>STAGKVIKCKAAVLWEEKKPFSIEEVEVAPPKAHEVRIKMVATGICRSDDHVVSGTLVTPLPVIAGHEAAGIVESIGEGVTTVRPGDKVIPLFTPQCGKCRVCKHPEGNFCLKNDLSMPRGTMQDGTSRFTCRGKPIHHFLGTSTFSQYTVVDEISVAKIDAASPLEKVCLIGCGFSTGYGSAVKVAKVTQGSTCAVFGLGGVGLSVIMGCKAAGAARIIGIDINKDKFAKAKEVGATECVNPQDYKKPIQEVLTEMSNGGVDFSFEVIGRLDTMVTALSCCQEAYGVSVIVGVPPDSQNLSMNPMLLLSGRTWKGAIFGGFKSKDSVPKLVADFMAKKFALDPLITHVLPFEKINEGFDL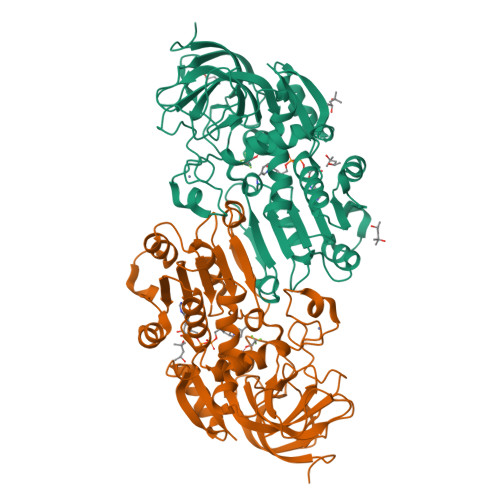LRSGESIRTILTF[2x]Baculovirus Autographa californica multiple nucleopolyhedrovirus (AcMNPV) has been widely used as a bioinsecticide and a protein expression vector. The DNA genome, along with the baculovirus basic DNA-binding protein P6.9 protein, is encapsulated by an enveloped, rod-shaped nucleocapsid; the major capsid protein VP39 and some additional minor proteins are known to comprise the nucleocapsid. Here, we show a 3.2 Å resolution structure of helical cylindrical body of the AcMNPV nucleocapsid, composed of VP39, as well as 4.3 Å resolution structures of both the head and the base of the nucleocapsid composed of over 100 protein subunits. Surprisingly, the C14 symmetric base had nearly identical features to that of the apical head, except for that in the central regions. Both the head and base could be further segmented into three parts: an outer shell, an inner layer and a central region.

At both ends of the nucleocapsid, the VP39 cylinder is constricted by an outer shell ring composed of proteins AC104, AC142 and AC109. Along the helical cylinder at the base (or head), three AC104 (VP80) subunits bind to the outer surface of VP39 at the end of the helical cylinder. AC109 sits adjacent to AC104-3 on the end of the VP39 helical cylinder and sterically blocks the elongation of the cylinder. AC109 appears to alter the conformation of the Thr163-Glu176 loop, elongating the “spine helix” in P-domain of VP39s at the terminal layer of the cylinder at both ends. This results in the formation of a disulfide bond between Cys169 of VP39 and Cys187 of AC109. Additionally, AC142 extensively interacts with a neighboring AC109 through a number of hydrogen bonds and salt bridges. These interactions result in fourteen AC109-AC142 hetero-dimers forming a “barrel-hoop” like structure, which tightens and constricts the capsid cylinder from 500 Å to ~400 Å in diameter. The inner layer of both the head and base is composed of AC101 and AC144 arranged with C14 symmetry. Interestingly, residues Leu243-His334 from each AC101, which is comprised of four helices and connecting loops, form a ring-like structure that encircles both AC144s in the inner layer. AC98 (38 K) is only found in the base as no discernable density corresponding to it can be found in the head. The N-terminal domain of AC98 interacts with VP39 and AC144, while also associating with genomic dsDNA. The interactions between AC101-2 and AC109 essentially bind the inner layer to the outer shell at both ends of the capsid.

>MNDSNSLLITRLAAQILSRNMQTVDVIVDDKTLSLEEKIDTLTSMVLAVNSPPQSPPRVTSSDLAASIIKNNSKMVGNDFEMRYNVLRMAVVFVKHYPKYYNETTAGLVAEIESNLLQYQNYVNQGNYQNIEGYDSLLNKAEECYVKIDRLFKESIKKIMDDTEAFEREQEAERLRAEQTAANALLERRAQTSADDVVNRADANIPTAFSDPLPGPSAPRYMYESSESDTYMETARRTAEHYTDQDKDYNAAYTADEYNSLVKTVLLRLIEKALATLKNRLHITTIDQLKKFRDYLNSDADAGEFQIFLNQEDCVILKNLSNLASKFFNVRCVADTLEVMLEALRNNIELVQPESDAVRRIVIKMTQEIKDSSTPLYNIAMYKSDYDAIKNKNIKTLFDLYNDRLPINFLDTSATSPVRKTSGKRSAEDDLLPTRSSKRANRPEINVISSEDEQEDDDVEDVDYEKESKRRKLEDEDFLKLKALEFSKDIVNEKLQKIIVVTDGMKRLYEYCNCKNSLETLPSAANYGSLLKRLNLYNLDHIEMNVNFYELLFPLTLYNDNDNSDKTLSHQLVNYIFLASNYFQNCAKNFNYMRETFNVFGPFKQIDFMVMFVIKFNFLCDMRNFAKLIDELVPNKQPNMRIHSVLVMRDKIVKLAFSNLQFQTFSKKDKSRNTKHLQRLIMLMNANYNVI[3x];> MECPFQIQVCISDRFFAFPHNLVEPQSDVGNKLIENLIVYVPTDDDRLYIDKKQFPKFNSVLVYRHEHDVNIDSRSPKKTASATIVYWNPLVPITEIGAGETRVFSVLLTNNLFYCNTMIVHHENPKCPIEFTYPETDMQSACSALLKNRNGQSVPPPIKSNLRPIACEIPLSHFKELVESNDFLLCFNLETSTMVKILSLKRIFCIFQYRKQPARYVINLPHEEIDNLYNKLNWERTRRLMKGDVPSNCATVNRSSLKYIKQAQSLLGIPDYSQTVVDFVKMFQKIIFPYQLVPNVIIKLNNFDQMVSSAPNKAEPYKKIRLFCKNDSIAISSSGIVPINMPDFSPPNTFDYSDYANRTNINFVTQRVLTDGGFSSGITVTPVKYNYYL;> MSGGGNLLTLERDHFKYLFLTSYFDLKDNEHVPSEPMAFIRNYLNCTFDLLDDAVLMNYFNYLQSMQLKHLVGSTSTNIFKFVKPQFRFVCDRTTVDILEFDTRMYIKPGTPVYATNLFTSNPRKMMAFLYAEFGKVFKNKIFVNINNYGCVLAGSAGFLFDDAYVDWNGVRMCAAPRLDNNMHPFRLYLLGEDMAKHFVDNNILPPHPSNAKTRKINNSMFMLKNFYKGLPLFKSKYTVVNSTKIVTRKPNDIFNEIDKELNGNCPFIKFIQRDYIFDAQFPPDLLDLLNEYMTKSSIMKIITKFVIEENPAMSGEMSREIILDRYSVDNYRKLYIKMEITNQFPVMYDHESSYIFVSKDFLQLKGTMNAFYAPKQRILSILAVNRLFGATETIDFHPNLLVYRQSSPPVRLTGDVYVVDKNEKVFLVKHVFSNTVPAYLLIRGDYESSSDLKSLRDLNPWVQNTLLKLLIPDSVQ;>MSAIALYLEINKLRLKIDEPMQLAIWPQLFPLLCDEHQSVQLNTDVLINFMMHVARKSQNTILNNNAAIASQYAAGNADVVAAPASAQPTPRPVINLFARANAAAPAQPSEELINMRRYRNAARKLIHHYSLNSTSSTEYKISDVVMTMIFLLRSEKYHSLFKLLETTFDDYTCRPQMTQVQTDTLLDAVRSLLEMPSTTIDLTTVDIMRSSFARCFNSPIMRYAKIVLLQNVALQRDKRTTLEELLIERGEKIQMLQPQQYINSGTEIPFCDDAEFLNRLLKHIDPYPLSRMYYNAANTMFYTTMENYAVSNCKFNIEDYNNIFKVMENIRKHSNKNSNDQDELNIYLGVQSSNAKRKKY[2x];>MKRIKCNKVRTVTEIVNSDEKIQKTYELAEFDLKNLSSLESYETLKIKLALSKYMAMLSTLEMTQPLLEIFRNKADTRQIAAVVFSTLAFIHNRFHPLVTNFTNKMEFVVTETNDTSIPGEPILFTENEGVLLCSVDRPSIVKMLSREFDTEALVNFENDNCNVRIAKTFGASKRKNTTRSDDYESNKQPNYDMDLSDFSITEVEATQYLTLLLTVEHAYLHYYIFKNYGVFEYCKSLTDHSLFTNKLRSTMSTKTSNLLLSKFKFTIEDFDKINSNSVTSGFNIYNFNK[2x];> MASSLQSKWICLRLNDAIIKRHVLVLSEYADLKYLGFEKYKFFEYVIFQFCNDPQLCKIIENNYNYCMQIFKAPADDMRDIRHNIKRAFKTPVLGHMCVLSNKPPMYSFLKEWFLLPHYKVVSLKSESLTWGFPHVVVFDLDSTLITEEEQVEIRDPFVYDSLQELHEMGCVLVLWSYGSRDHVAHSMRDVDLEGYFDIIISEGSTVQEERSDLVQNSHNAIVDYNLKKRFIENKFVFDIHNHRSDNNIPKSPKIVIKYLSDKNVNFFKSITLVDDLPTNNYAYDFYVKVKRCPTPVQDWEHYHNEIIQNIMDYEQYFIK;>MALVPVGMAPRQMRVNRCIFASIVSFDACITYKSPCSPDAYHDDGWFICNNHLIKRFKMSKMVLPIFDEDDNQFKMTIARHLVGNKERGIKRILIPSATNYQDVFNLNSMMQAEQLIFHLIYNNENAVNTICDNLKYTEGFTSNTQRVIHSVYATTKSILDTTNPNTFCSRVSRDELRFFDVTNARALRGGAGDQLFNNYSGFLQNLIRRAVAPEYLQIDTEELRFRNCATCIIDETGLVASVPDGPELYNPIRSSDIMRSQPNRLQIRNVLKFEGDTRELDRTLSGYEEYPTYVPLFLGYQIINSENNFLRNDFIPRANPNATLGGGAVAGPAPGVAGEAGGGIAV[4x]>WSKCNPLEKTCPPNK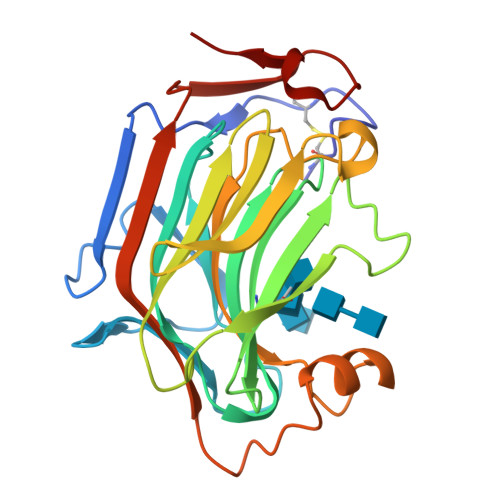GLAASTYTADFTSASALDQWEVTAGKVPVGPQGAEFTVAKQGDAPTIDTDFYFFFGKAEVVMKAAPGTGVVSSIVLESDDLDEVDWEVLGGDTTQVQTNYFGKGDTTTYDRGTYVPVATPQETFHTYTIDWTKDAVTWSIDGAVVRTLTYNDAKGGTRFPQTPMRLRLGSWAGGDPSNPKGTIEWAGGLTDYSAGPYTMYVKSVRIENANPAESYTYSDNSGSWQSIKFD[2x]Slow bee paralysis virus (SBPV) belongs to the Iflaviridae family of nonenveloped single-stranded RNA viruses. The overall structure of the virion resembles that of picornaviruses, with the three major capsid proteins VP1 to 3 organized into a pseudo-T3 icosahedral capsid. However, the SBPV capsid protein VP3 contains a C-terminal globular domain that has not been observed in other viruses from the order Picornavirales. Furthermore, the P domain contains the Ser-His-Asp triad within a surface patch of eight conserved residues that constitutes a putative catalytic or receptor-binding site.

The two structures are similar, with a Cα-atom root mean square deviation (RMSD) of 0.27 Å; however, they differ in the positions of protruding (P) domains of the VP3 subunits on the virion surface. In crystal form 1, five P domains related by one icosahedral 5-fold axis form a “crown” on the virion surface. The crowns have a diameter of 90 Å and protrude 50 Å above the capsid surface, giving the SBPV virion its characteristic shape. Residues from loop β2-β3 as well as the N- and C-terminal loops and β2 of the P domain interact with the BC, CD, and EF loops of VP1, forming an interface with a buried surface area of 850 Å2. P domains within the same crown do not interact with each other. In crystal form 1, the electron density map corresponding to the P domains is less well ordered than that of the rest of the SBPV virion, indicating an increased mobility of the crown. The P domains are positioned in different locations on the virion surface in the two crystal forms. It is important to note that the domains are not held in position by crystal contact in either of the crystal forms. The crystallization conditions that produced the two crystal forms of SBPV differed in terms of solution components and pH, which was 6.5 for crystal form 1 and 4.5 for crystal form 2. We speculate that the differences in localization of the P domains might be induced by the differences in the crystallization conditions. The GH loop is exposed on the virion surface in crystal form 1 but is partly covered by the P domain in crystal form 2.

> MERTFTPNVMQPTPLLPTTNDGRVTFGEAFNDLKDLARRYQLYWEGTILEGNLRAIRRNSALVQLPLYPHGLRIQPDVNNPIWNIMRDGHIPVISSGFRYFRGGLRLRIVVEGLNSCVWVQHHPDRPSIFSRPIIGRYIAAKDAYRNHAYAAYVQNMSVNRTIEVEVPFYQPGLYGMLNASDNNTANSFDRLRFTGLGDLLIGIEGEQPIPKEGIEISVYYSIADDFSFNIFCGFPPMVYCDETYSAATPDLAQYFEDEVTIAQPE;> MDRPEGSEERTVQTSNVVLGETNIESQDIASKEYSPTWDRLASSEVSDEYPMLTDRWLFWKSVKWEVNDSAFGKMLVQEKFPQSWVQMDVNVNNIPRYTNIPNFIPFNIHQYMRADFEVKIYVNPNDFVSGWLIMAFLYQGSEMFDYKLRRNPAALMQMPHVLVNVGAANEATLKIPYRYVRPFMRCKDILRGDNLITGVTEPLNMGVLFVEVLIPFRTSAASSAPKSLDVSLFVKMTNAKFTGMVDGSIALLSKPIALPE;> DNPPDPTPAKFFVPIPSHSWAHGTNTSEPTNTLRLDGGVVGVGRSDDIGTSDTAISGIIGVYGLLKPFDWNANDTGRNVGGHLLWSMPVHPQVDKDQVIQVMTQSKLTQYYLPPISVVSSLYAYTRGSIKYKFLFGNNPRHNARLLVAYIPGISSDNRLTLERARNSAHVVFSLNEVSEFVFTVPYITDTMWWPRKYGGPQAAGEFVAPSYICMFILNPLVAMESVPSIVTIVPMIAAGDDFEVAVPAQPAVGLSRNIDVIYPKDSIISFKSGYFPVYVGSWHSFFDSTKAILRYGAVSDHIAQLGNIPANVNRKAFWIVVGDTIKFKTKLDKINGTEWFIPEGEYTLGYGVVWRDGAYAYMVPYPLTPLGEKIAQYTASLLASNTAISQIRPYIPDYIVDSAASKDNILWSPIEDRLRAQTEWVMAEPE>SEFELGAPAGRQAGQQATVDRLRTQVTGFLSGALGKLQALSAQNMDPELAQFRVLDVDRAIMPLLIVAENARNPGLNLVPLHMDMAEDEEVRTQPPMAGSRHIAEFVASARPGRYRAVIDDGSHTRAADIRKDASGTSVIVVDPLRKEKDESAYVDYADNVNMEFGEHAKCAFIPVDIQKSSFDCRILSLSLALKMHDKDDAFAAFHETLRNGGDPSHHVSRAQQTEELGATLVLDGAPLVDARMMKHGQAASSVSRYLGNHPEQSTVPVNKRNETLGERTTRHLVKRKVRNRADSEGRVTSGETKEITFSNSVEQKRIALLNRAASYVNSAPPPVVMRMAKLLQDSLL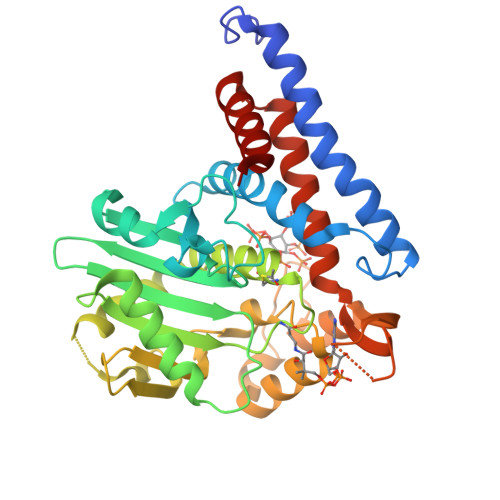DTN[4x]> ETTQKLTVSHIEGYECQPIFLNVLEAIEPGVVCAGHDNNQP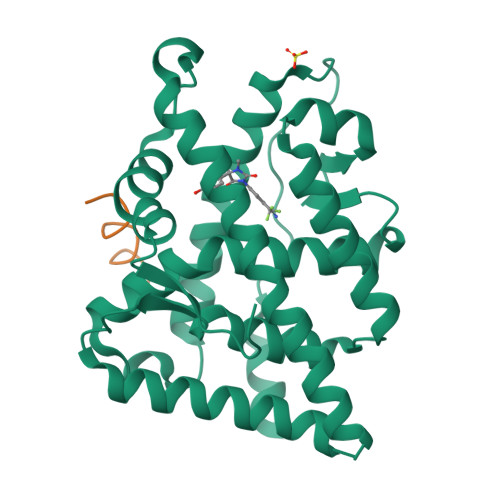DSFAALLSSLNELGERQLVHVVKWAKALPGFRNLHVDDQMAVIQYSWMGLMVFAMGWRSFTNVNSRMLYFAPDLVFNEYRMHKSRMYSQCVRMRHLSQEFGWLQITPQEFLCMKALLLFSIIPVDGLKNQKFFDELRMNYIKELDRIIACKRKNPTSCSRRFYQLTKLLDSVQPIARELHQFTFDLLIKSHMVSVDFPEMMAEIISVQVPKILSGKVKPIYFHTQ;> GAFQNLFQSVR>MASRGSHHHHHHGAYRLLNKTAVITGGNSGIGLATAKRFVAEGAYVFIVGRRRKELEQAAAEIGRNVTAVKADVTKLEDLDRLYAIVREQRGSIDV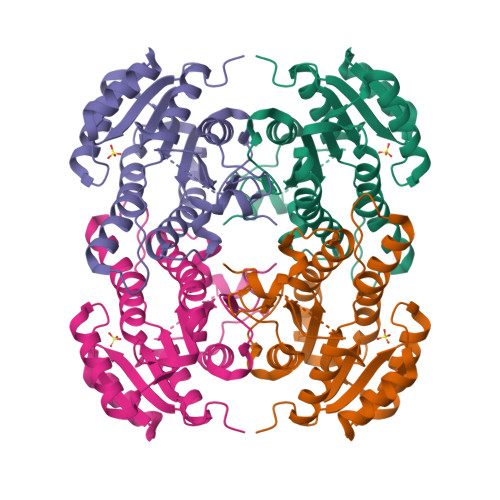LFANSGAIEQKTLEEITPEHYDRTFDVNVRGLIFTVQKALPLLRDGGSVILTSSVAGVLGLQAHDTYSAAKAAVRSLARTWTTELKGRSIRVNAVSPGAIDTPIIENQVSTQEEADELRAKFAAATPLGRVGRPEELAAAVLFLASDDSSYVAGIELFVDGGLTQV[8x]> MGHHHHHHMIEWIIRRSVANRFLVLMGALFLSIWGTWTIINTPVDALPDLSDVQVIIKTSYPGQAPQIVENQVTYPLTTTM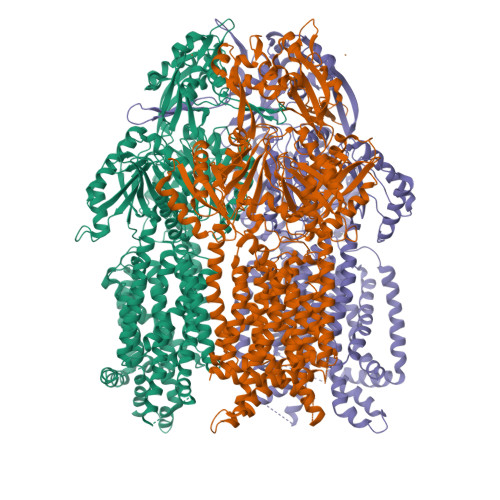LSVPGAKTVRGFSQFGDSYVYVIFEDGTDPYWARSRVLEYLNQVQGKLPAGVSAELGPDATGVGWIYEYALVDRSGKHDLADLRSLQDWFLKYELKTIPDVAEVASVGGVVKEYQVVIDPQRLAQYGISLAEVKSALDASNQEAGGSSIELAEAEYMVRASGYLQTLDDFNHIVLKASENGVPVYLRDVAKVQIGPEMRRGIAELNGEGEVAGGVVILRSGKNAREVIAAVKDKLETLKSSLPEGVEIVTTYDRSQLIDRAIDNLSGKLLEEFIVVAVVCALFLWHVRSALVAIISLPLGLCIAFIVMHFQGLNANIMSLGGIAIAVGAMVDAAIVMIENAHKRLEEWQHQHPDATLDNKTRWQVITDASVEVGPALFISLLIITLSFIPIFTLEGQEGRLFGPLAFTKTYAMAGAALLAIVVIPILMGYWIRGKIPPESSNPLNRFLIRVYHPLLLKVLHWPKTTLLVAALSVLTVLWPLNKVGGEFLPQINEGDLLYMPSTLPGISAAEAASMLQKTDKLIMSVPEVARVFGKTGKAETATDSAPLEMVETTIQLKPQEQWRPGMTMDKIIEELDNTVRLPGLANLWVPPIRNRIDMLSTGIKSPIGIKVSGTVLADIDAMAEQIEEVARTVPGVASALAERLEGGRYINVEINREKAARYGMTVADVQLFVTSAVGGAMVGETVEGIARYPINLRYPQSWRDSPQALRQLPILTPMKQQITLADVADIKVSTGPSMLKTENARPTSWIYIDARDRDMVSVVHDLQKAIAEKVQLKPGTSVAFSGQFELLERANHKLKLMVPMTLMIIFVLLYLAFRRVGEALLIISSVPFALVGGIWLLWWMGFHLSVATGTGFIALAGVAAEFGVVMLMYLRHAIEAVPSLNNPQTFSEQKLDEALYHGAVLRVRPKAMTVAVIIAGLLPILWGTGAGSEVMSRIAAPMIGGMITAPLLSLFIIPAAYKLMWLHRHRVRK N-oxalyl-alpha-methylalanine 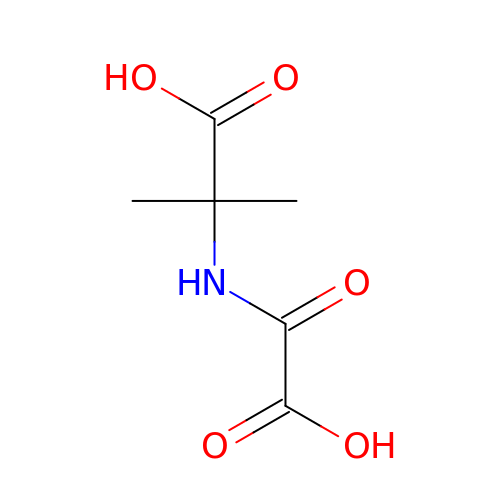| C6 H9 N O5 | ISTWWSBLMQHYIQ-UHFFFAOYSA-N>[2x]DRHHHHHHKLSRAH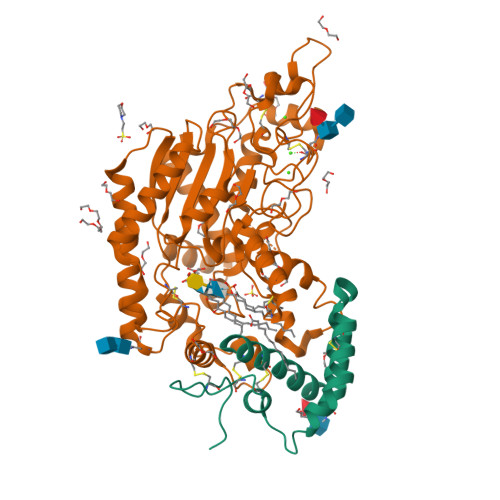DNQPGTIRSDHYTCVGCVLVVSVIEQLAQVHNSTVQASMERLCSYLPEEWVLKTACYMMVHVFGADIIKLFDKDVNADVVCHTLEFCKQEPGQPLCHLYPLPKESWKFTLEKARHIVKQSPIMKYTR;>[2x]SGAGICSLPFLAKICQKIKLAIKNSVPIKDVDSDKYSIFPTLRGYHWRGRDCNDSDKTVYPGRRPDNWDAHRDSNCNGIWGVDPKDGIPYEKKFCEGSQPRGIILLGDAAGAHFHIPPEWLTVSQMSVNSFLNLPTAVTNELDWPQLSGTTGFLDSASKIKENSIYLRLRKRNRCNHRDYQNISKNGASSRNVKSLIESLSRNQLLDHPAIVIYAMIGNDVCNGRKTDPVSAMTTPEQLYANVLKMLEALNSHLPTGSHVILYGLAHGAFLWDTLHSRYHPLGQLNKDVTYTQLYSFLGCLQVSPCPGWMSANETLRALTSERAQQLSETLRKIAASKKFTNFNLFYLDFAFQEVVEEWQKMGGQPWELIEAVDGFHPNEVALLLFADQLWEKVQRQWPDVLGKENPFNPQIEEVFGDQGGH(3~{S})-1-[4-chloranyl-3-(trifluoromethyl)phenyl]pyrrolidine-3-carboxylic acid | C12 H11 Cl F3 N O2 | 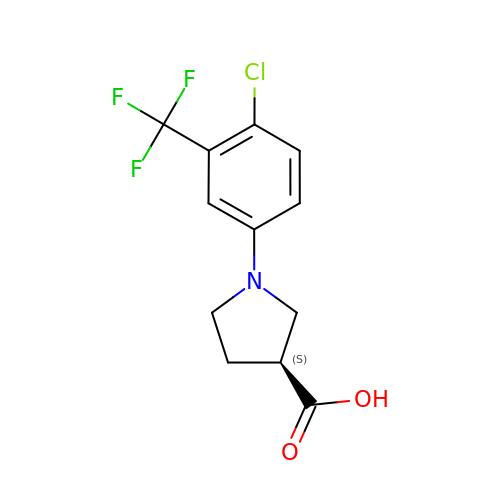XTYYFZCQCKEYKG-ZETCQYMHSA-N>[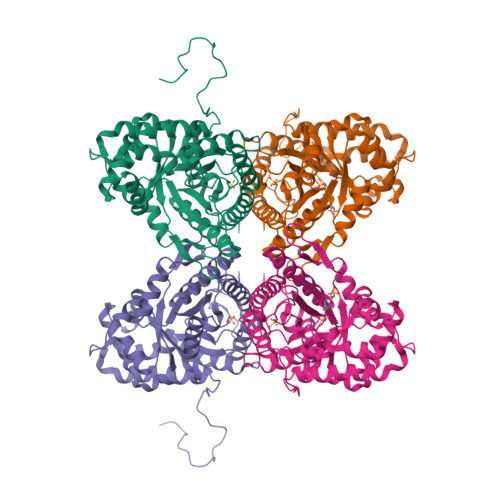4x]AHRFPALTPEQKKELSDIAQRIVANGKGILAADESVGTMGNRLQRIKVENSEENRRQFREILFTVDNSINQSIGGVILFHETLYQKDSQGKLFRNILKEKGIVVGIKLDQGGAPLAGTNKETTIQGLDGLSERCAQYKKDGVDFGKWRAVLRIADQCPSSLAIQENANTLARYASICQQNGLVPIVEPEVIPDGDHDLEHCQYVTEKVLAAVYKALNDHHVYLEGTLLKPNMVTAGHACTKKYTPEQVAMATVTALHRTVPAAVPGICFLSGGMSEEDATLNLNAINLCPLPKPWKLSFSYGRALQASALAAWGGKAENKKATQEAFMKRAVVNCQAAKGQYVHTGSSGAASTQSLFTASYTY> GSVDDSAQSDLKEVMVLNATESFVYEPKEQKKMFHATVATENEVFRVKVFNIDLKEKFTPKKIIAIANYVCRNGFLEVYPFTLVADVNADRNMEIPKGLIRSASVTPKINQLCSQTKGSFVNGVFEVHKKNVRGEFTYYEIQDNTGKMEVVVHGRLTTINCEEGDKLKLTCFELAPKSGNTGELRSVIH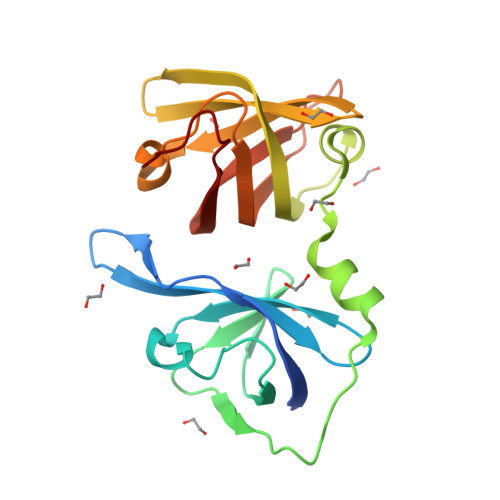SHIKVIKTRKNAAAS4-[[(3S,4S,5R)-4-(hydroxymethyl)-5-(3-methoxy-4-oxidanyl-phenyl)oxolan-3-yl]methyl]-2-methoxy-phenol | C20 H24 O6 | 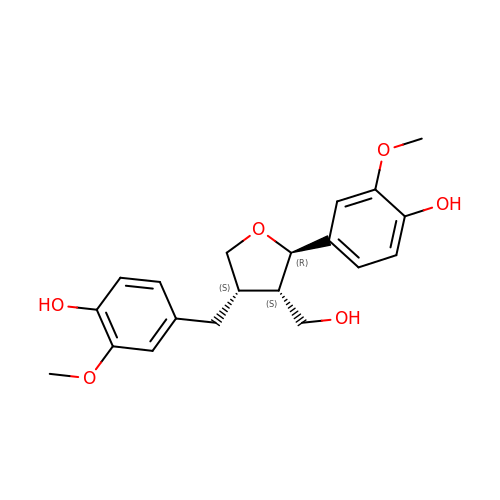MHXCIKYXNYCMHY-SXGZJXTBSA-N> MPREIITLQLGQCGNQIGFEFWKQLCAEHGISPEGIVEEFATEGTDRKDVFFYQADDEHYIPRAVLLDLEPRVIHSILNSPYAKLYNPENIYLSEHGGGAGNNWASGFSQGEKIHEDIFDIIDREADGSDSLEGFVLCHSIAGGTGSGLGSYLLERLNDRYPKKLVQTYSVFPNQDEMSDVVVQPYNSLLTLKRLTQNADCVVVLDNTALNRIATDRLHIQNPSFSQINQLVSTIMSASTTTLRYPGYMNN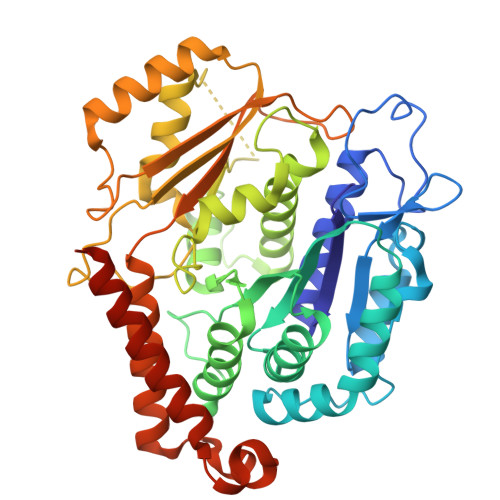DLIGLIASLIPTPRLHFLMTGYTPLTTDQSVASVRKTTVLDVMRRLLQPKNVMVSTGRDRQTNHCYIAILNIIQGEVDPTQVHKSLQRIRERKLANFIPWGPASIQVALSRKSPYLPSAHRVSGLMMANHTSISSLFESSCQQYDKLRKREAFLEQFRKEDIFKENFDELDRSREVVQELIDEYHAATRPDYISWGTQEQ> MGSSHHHHHHSQDLEVLFQGPHMAFEKPLRKLTFADLLQATNGFHNDSLIGSGGFGDVYKAILKDGSAVAIKKLIHVSGQGDREFMAEMETIGKIKHRNLVPLLGYCKVGDERLLVYEFMKYGSLEDVLHDPKKAGVKLNWSTRRKIAIGSARGLAFLHHNCSPHIIHRDMKSSNVL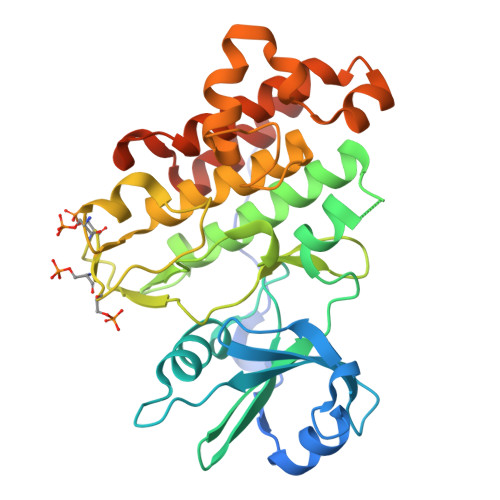LDENLEARVSDFGMARLMSAMDTHLSVSTLAGTPGYVPPEYYQSFRCSTKGDVYSYGVVLLELLTGKRPTDSPDFGDNNLVGWVKQHAKLRISDVFDPELMKEDPALEIELLQHLKVAVACLDDRAWRRPTMVQVMAMFKEIQAGSGIDSQSTIRS>MQSINFRTARGNLSEVLNNVEAGEEVEITRRGREPAVIVSKATFEAYKKAALDAEFASLFDTLD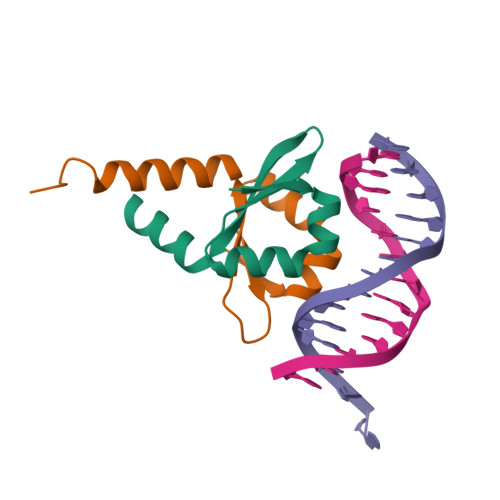STNKELVNR[4x]>MSVTVPNDDWTLSSLSETFDDGTQTLQGELTLALDKLAKNPSNPQLLAEYQSKLSEYTLYRNAQSNTVKVIKD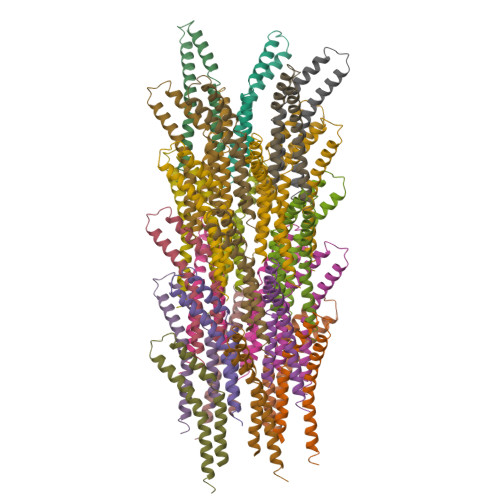VDAAIIQNFR[28x]> MEANGLGPQGFPELKNDTFLRAAWGEETDYTPVWCMRQAGRYLPEFRETRAAQDFFSTCRSPEACCELTLQPLRRFPLDAAIIFSDILVVPQALGMEVTMVPGKGPSFPEPLREEQDLERLRDPEVVASELGYVFQAITLTRQRLAGRVPLIGFAGAPWTLMTYMVEGGGSSTMAQAKRWLYQRPQASHQLLRILTDALVPYLVGQVVAGAQALQLYESHAGHLGPQLFNKFALPYIRDVAKQVKARLRE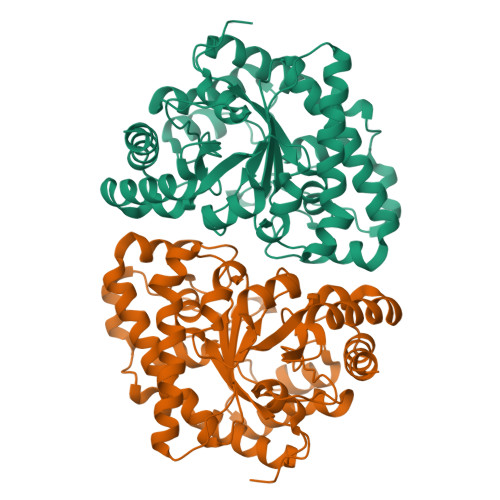AGLAPVPMIIFAKDGHFALEELAQAGYEVVGLDWTVAPKKARECVGKTVTLQGNLDPCALYASEEEIGQLVKQMLDDFGPHRYIANLGHGLYPDMDPEHVGAFVDAVHKHSRLLRQN>[6x]APPCSRCFARAIESSRDLLHRIKDEVGAPGIVVGVSVDGKEVWSEGLGYADVENRVPCKPETVMRIASISKSLTMVALAKLWEAGKLDLDIPVQHYVPEFPEKEYEGEKVSVTTRLLISHLSGIRHYEKDIKKVKEEKAYKALKMMKENVAFEQEKEGKSNEKNDFTKFKTEQENEAKCRNSKPGKKKNDFEQGELYLREKFENSIESLRLFKNDPLFFKPGSQFLYSTFGYTLLAAIVERASGCKYLDYMQKIFHDLDMLTTVQEENEPVIYNRARFYVYNKKKRLVNTPYVDNSYKWAGGGFLSTVGDLLKFGNAMLYGYQVGLFKNSNENLLPGYLKPETMVMMWTPVPNTEMSWDKEGKYAMAWGVVERKQTYGSCRKQRHYASHTGGAVGASSVLLVLPEELDTETINNKVPPRGIIVSIICNMQSVGLNSTALKIALEFDKDRSD

In mitochondria, the serine beta-lactamase-like protein (LACTB), which is localized in mitochondrial IMS, functions as a tumor suppressor by regulating the PE biosynthetic pathway. LACTB is a conserved mammalian active-site serine protease present in all vertebrates. The conserved catalytic serine residue within the 164SXXK167 motif plays an important role in the enzymatic activity of LACTB and is reversibly acylated through substrate binding. Mammalian LACTB is localized in the mitochondrial intermembrane space (IMS), where it assembles into filaments to regulate the efficiency of essential metabolic processes.

To examine the molecular architecture of human LACTB, we purified near full-length LACTB (residues 97 to 547) lacking the N-terminal targeting sequence. A final cryoEM reconstruction of the LACTB filament was obtained at an overall resolution of 3.1 Å with an imposed helical symmetry. Further analysis of the structural data revealed that the basic building blocks of LACTB are dimers, which are stacked on each other and assembled into filaments with a helical twist of 48.25° and a rise of 21.63 Å. LACTB has a globular structure with approximate dimensions of 60 Å × 55 Å × 45 Å and consists of a five-stranded β-sheet core (β1, β2, β7, β8, and β9) surrounded by 2 short two-stranded antiparallel β-sheets (β3 - β4 and β5 - β6) and 10 α-helices (α1 - α10). Our 3.1 Å map also enabled the identification of the amino acid motifs (164SISK167, 323YST325, and 485HTG487) that contribute to the formation of the catalytic site, including the catalytic S164 residue, all of which are conserved across metazoan species. The LACTB filaments assemble as stacked antiparallel dimers, where the buried surface area between the two protomers (A and B) is approximately 945 Å2. Assembly of the LACTB dimer is mediated by the combined effects of sixteen hydrogen bond interactions between E149, N150, N364, E365, P366, I368, N370, R371, N385, and T386 residues and two inter-molecular salt bridges between E149 and R371. The inspection of the inter-dimer interface shows that three assembly contacts between neighboring subunits (A and C, A and D, and B and D) bridge antiparallel LACTB homodimers and drive filament assembly. The first polymer interface, which spans a buried solvent-accessible surface area of approximately 780 Å2, is formed between the α1 helix and L3 along with the protruding L10 loop between β3 and β4 strands of protomers A and D. The filament structure also shows a second polymer interface that has symmetric contact sites between protomers A and C and B and D, which bury approximately 540 Å2 of solvent-accessible surface area.>GSHMLSIYQDQEQRILKFLEELGEGKATTAHDLSGKLGTPKKEINRVLYSLAKKGKLQKEAGTPPLWKIAVSTQAWNQHSG[3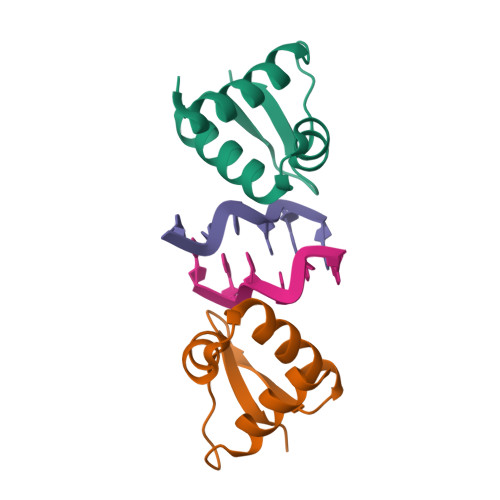x]>MNKPVKKQQPKKVIPNFEYARRLNG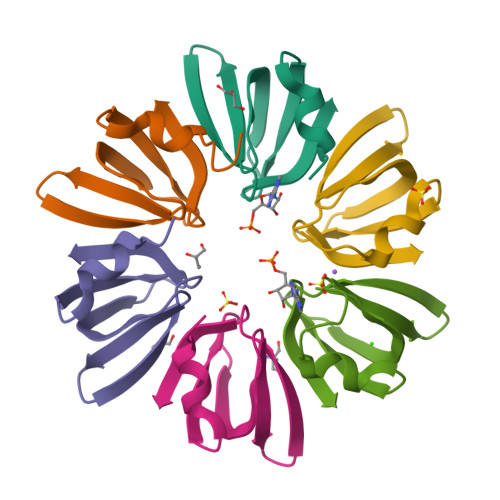KKVKIFLRNGEVLDAEVTGVSNYEIMVKVGDRNLLVFKHAIDTIEY[12x]> GVIDTSAVESAITDGQGDMKA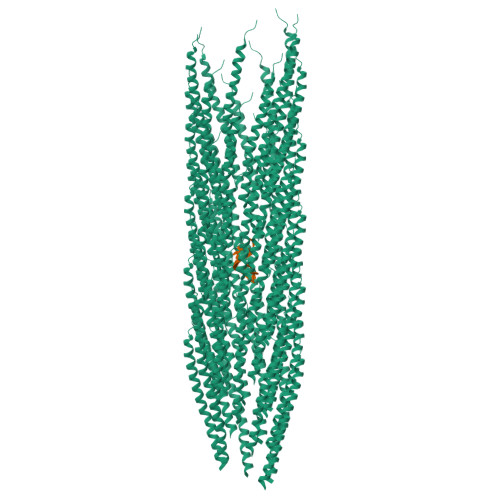IGGYIVGALVILAVAGLIYSMLRKA The well-studied Siphovirus T5 has a three-fold symmetric tail-tube, to the end of which three long, L-shaped fibres are attached. These fibres are made up of a homotrimer of protein pb1 (pb stands for “protein band”). The L-shaped tail fibres are responsible for the initial recognition of certain Escherichia coli (E. coli) host strains, binding to the O8- or O9-type O-antigen of the bacterial lipopolysaccharide (LPS). The bacteriophage T5 L-shaped tail fibre uses an intra-molecular chaperone to fold, which is then auto-proteolytically released to yield the mature protein.

A single point mutation (T to G), mutating the codon of the corresponding serine in pb1 (Ser1264) to code for alanine, was introduced into the plasmid pET-28-pb1(970–1396). Expression of the mutated gene in E. coli cells led to production of the non-proteolyzed version of the protein, which we call pb1(970–1396). The resulting model was used to phase the structure of pb1(970–1396) by molecular replacement. Three trimers were located in the asymmetric unit, and the intra-molecular chaperone region could be constructed by a combination of automated and manual building in the calculated electron density. Serine 1264, the residue responsible for the auto-proteolytic cleavage of the carboxy-terminal domain from the bullet-shaped domain, is located between the bullet-shaped and intra-molecular chaperone domains. In the structure where Ser1264 has been substituted with alanine, the chain continues with a loop (residues 1265–1276) winding around the other three, subsequently forming a hairpin (residues 1277–1322). Three 50 Å-long hairpins (residues 1332–1371 from each monomer, containing beta-strands C' through F', protrude upwards and embrace the preceding bullet-shaped domain). The intra-molecular chaperone domain (ic) ends in a central triple-helical coiled-coil, to which each monomer contributes their carboxy-terminal alpha-helix (formed by residues 1371–1394). In the structure with the chaperone, two short beta-strands are present in the third interdigitated region, forming a four-stranded beta-sheet with the C′ and F′ beta-strands of the chaperone domain. Although the interface between the bullet-shaped domain and the intra-molecular chaperone domain appears extensive, it is only 3 × 103 Å2 large and the association is accompanied by a free energy gain of just −12 kcal/mol.

>ETTATTGIGVNFIGDSATECSFGIENTAGGSAVFHNYTRGASNSVTKNNQLLGGYGSRPWLGSTYTEHSNAALHFLGAGDTSATNHGGWIRLLVTPKGKTISDRVPAFRLSDNGDLWLVPDGAMHSDLGLVRSIETLNAAVPRFNAPSIQDGRGLKIVAPQAPEIDLIAPRGSGASAPAIRAMWCDGSLADTTRYIGATQPGSTFYIGASGHDGEKFDSMRGSVAIKSAGGWGPTSTPTQVVLETCESGSISRLPRWGVDHNGTLMPMADNRYNLGWGSGRVKQVYAVNGTINTADARLKNDVRAMSDPETEAAKAIAKEIGFWTWKEQADMNDIREHCGLTVQRAIEIMESFGLDPFKYGFICYDKWDEHTVVSEYGPANEDGTENPIYKTIPAGDHYSFRLEELNLFIAKGFEARLSAIEDKLGM[9x]>[2x]MRGSHHHHHHGSSNTPQNVQLANFPSLKGKRVFITGGGTGIGAAIVEAFAQQGAHVAFVDIATEASEALCNDIAAAGHPKPLFRHCDLRDIPAFQATIAELQGQLGDFDVLVNNAANDQRHKLEEVTLEYWNDRIAINQRPSFFAVQSVVEGMKRRGGGSIINFSSISWHQSGGGFPVYTTAKASTLGLTRGLARDLGPH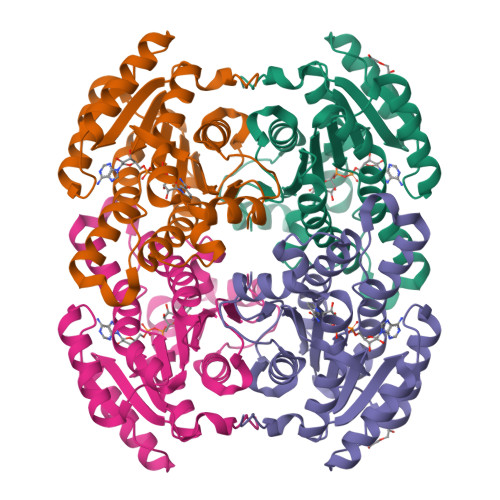KIRVNTVTPGWVMTERQIKLWLDEEGKKAIARNQCLQGDLLPWHLARMVLFLAADDSAMCTAQEFIVDAGWV>[2x]MGSSHHHHHHSSENLYFQGHSKSPRKDYAKLANYDESKVPQYTLPSVLMCHDGEMVQTKEQWEQKRRPEILNLFTTYMFGKAPVLKHKLPCTVSRINEKALNGRATRKEITIQLTDDPQGPHIDLQLY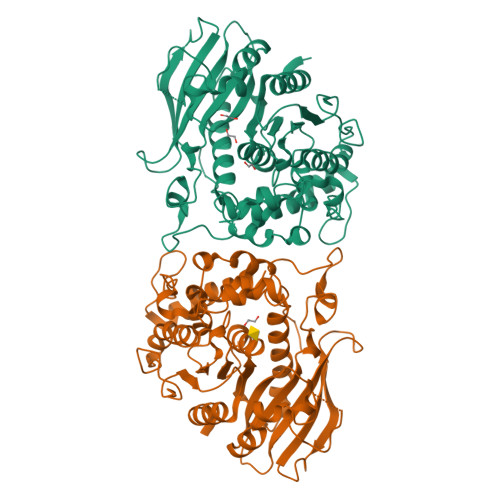LPNHVSGKIPVFLGISFMPNYTIYDDPDLSVPEITDEKMKKRSFRGSMDKSWQLDKILEHGYGLATFCYNDVDPDFDDDFQNGVHPYYYEKGQNFPDPDQWGSIAAWAWGMSRAMDYLETDKKVDAKKVAVIGHSRLGKTAVWAGASDPRFALVISGNSGCCGVAISRRCFGETVEAMNVRFPHWFCGNYKQFNDREKYLPFDQHELVALIAPRPIYIASAEEDNWSDQKGEFLGGKGAEPVYALYGLGGIGCEEMPPVDTPYMNGPIAYHNRKGPHAVLPYDWEQFLRFADKYFKNK>[2x]MKFNENFVWGVATSSYQIEGAYNEDGRGKDIWGDYCSIPGIIFDNHNGDKACEHYYRYKEDVAIMKEMGIKAYRFSIAWARIFPEGIGKINQKGVDFYHNLIDELIKNDIVPYVTLFHWDLPLELAEKGGWLNDDSVE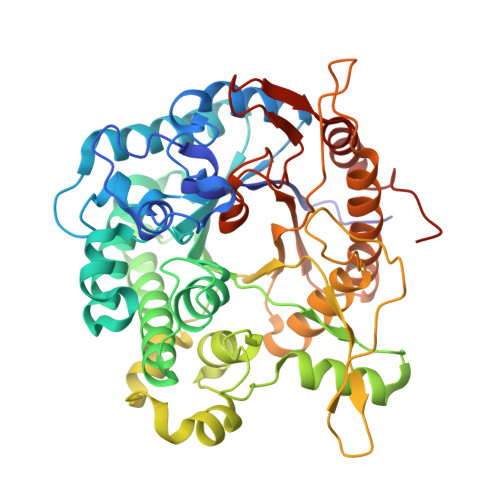WFKDYAEFFGKEYGHKIKYIMTFNEPQCTIGLGLQQGIHAPGVKLSPKAVLKSTHNLLKAHGAAVKVLRKVAPNTQLGIAPTCGVALPISENKKDIEIARKRYFDILDLNDAYVWSVSLFLDPIVLGDYPTKYYELYKEHLPKITQEDLKLISQPLDFLAQNIYNGYRVSEDENGNYVYPKRKAGYDHTDMGWPITPSALYWGPRFICERYNLPFYITENGLACHDVVSLDNKVHDPNRIDFLNKYLLDYSRASCEGYDIRGYFQWSLMDNFEWREGYSKRFGMVYVDFETQKRTIKDSGYWYKKVIEENGENLLEHHHHHH Here, we report a detailed characterization of AGa, an uncultured Bacteroidetes-affiliated genotype that is predicted to be cellulolytic, albeit via an unknown mechanism. Taking meta-omics and enzymology analyses into consideration, we propose a non-classical cellulose degradation mechanism that involves the utilization of multi-modular enzymes that are secreted via the Bacteroidetes-specific T9SS. All five GH5 domains in this cluster were affiliated to GH5 subfamily 2, the largest of the GH5 subfamilies. Enzymes in this family are mostly extracellular and are endo-acting β-1,4-glucanases.

Cel5C contains two GH5 domains (Cel5C_N and Cel5C_C) that have 45% sequence identity to each other, and low similarity to their closest homologues, which consisted of individual GH5 domains (from single GH-containing proteins) from the known cellulolytic Bacteroidetes species Sporocytophaga myxococcoides (40–50% sequence identity) and Saccharicrinis fermentans (38–56% sequence identity). Comparing specific activities revealed Cel5D and the individual N-terminal GH5 domain in Cel5C (Cel5C_N) as the most active. Interestingly, Cel5C_N outperformed the full-length Cel5C_wt, whereas the other GH5 domain, Cel5C_C, had too low activity on CMC to determine the specific activity. Similar to the relative activities on CMC, Cel5C_N and Cel5D were the most active, releasing mostly cellobiose and some glucose from Avicel. In comparison, Cel5C_N generated ~ 800 μM of cellobiose from 1% Avicel in 24 h. Cel5C_N and Cel5D were too active to show the stepwise degradation of Glc(5) or Glc(6) in the assayed time points, degrading both substrates to completion in 30 s. Both enzymes produced Glc(2) and Glc(3) from Glc(5), whereas Glc(6) was converted to a mixture dominated by Glc(2) but also containing Glc(3). The enzymes thus cleave Glc(6) by binding the substrate to subsites − 3 to + 3, producing Glc(3), and to − 4 to + 2 or − 2 to + 4, to produce Glc(4) which is further degraded to Glc(2). The inability of the otherwise highly active Cel5C_N to degrade decorated hemicellulose substrates (e.g. xyloglucan) was supported by structural characterization studies, which resolved the structure of Cel5C_N to 1.57 Å. The structure displays a (β/α)8-barrel fold, typical to GH5 enzymes, although a comparably narrower active-site cleft was observed, similar to that of GH5 enzymes that specifically accommodate linear polysaccharides, such as cellulose.

> TYPEGSPVYHNGKLSVQGTQMVSECGKPVQLRGMSSHGLAWFPKCYTEASLTALVKDWNIDIFRLAIYTHEWGGYTTNQWKSKDDYNAYIDNMVDICAKLGIYCIIDWHVLNDGSGDPNYTLDDAIPFWDYMSAKHKDDKHVLYEICNEPNGFDVKWADVKEYAEAVIPVIRKNDPDKIIICGTPTWSQDVDLAAQDPLSYDNVMYTLHFYSGTHTQYLRDKAQVAINKGLALFVTEFGTTQASGDGGVYFDECNTWMDWMDARKISWVNWSFADKPESSAALKPGASNSGDWNMVSESGQYIKRKLSQPKSYESCGGHHHHH> HMFDVVVIGGGISGLSAAKLLTEYGVSVLVLEARDRVGGRTYTIRNEHVDYVDVGGAYVGPTQNRILRLSKELGIETYKVNVSERLVQYVKGKTYPFRAAFPPVWNPIAYLDYNNLWRTIDNMGKEIPTDAPWEAQHADKWDKMTMKELIDKICWTKTARRFAYLFVNINVTSEPHEVSALWFLWYVKQCGGTTRIFSVTNGGQERKFVGGSGQVSERIMDLLGDQVKLNHPVTHVDQSSDNIIIETLNHEHYECKYVINAIPPTLTAKIHFRPELPAERNQLIQRLPMGAVIKCMMYYKEAFWKKKDYCGCMIIEDEDAPISITLDDTKPDGSLPAIMGFILARKADRLAKLHKEIRKKKICELYAKVLGSQEALHPVHYEEKNWCEEQYSGGCYTAYFPPGIMTQYGRVIRQPVGRIFFAGTETATKWSGYMEGAVEAGERAAREVLNGLGKVTEKDIWVQEPESKDVPAVEITHTFWERNLPSVSGLLKIIGFSTSVTALG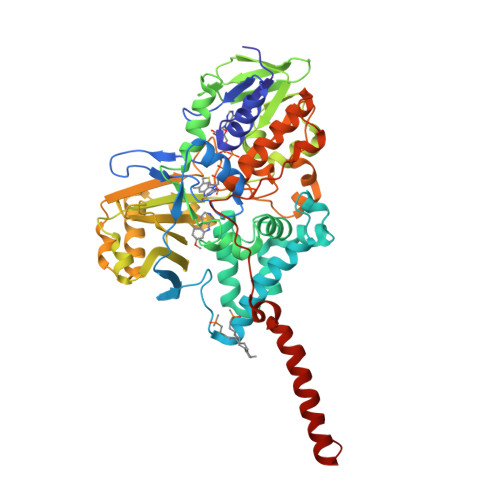FVLYKYKLL>QDINAQLTTWFSQRLAGFSDEVVVTLRSSPNLLPSCEQPAFSMTGSAKLWGNVNVVARCANEKRYLQVNVQATGNYVAVAAPIARGGKLTPANVTLKRGRLDQLPPRTVLDIRQIQDAVSLRDLAPGQPVQLTMIRQAWRVKAGQRVQVIANGEGFSVNAEGQAMNNAAVAQNARVRMTSGQ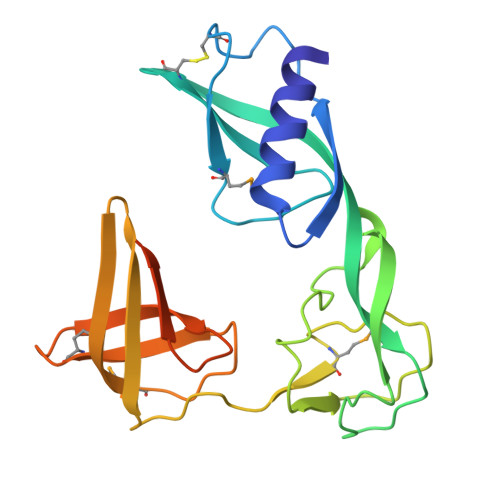IVSGTVDSDGNILINLDPNSSSVDKLAAALEHHHHHH[2x]> GSSRTSVQTEDDQLIAGQSAGSGSAQLPQEEKAKIAEQVEIFHQEKSKLDAEVAKWDDSGNDIIVLAKQMCMIMMEMTDFTRGKGPLKNTSDVINAAKKIAEAGSRMDKLARA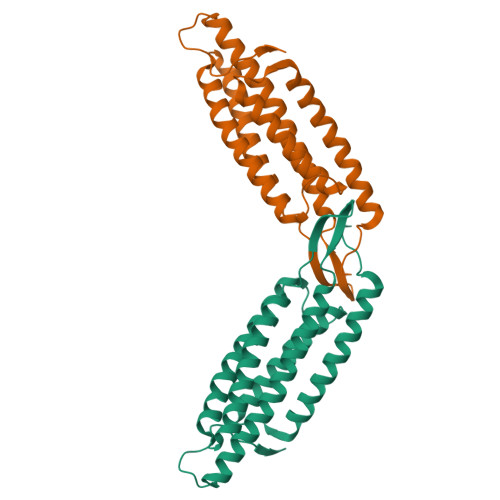VADQCPDSACKQDLLAYLQRIALYCHQLNICSKVKAEVQNLGGELIVSGLDSATSLIQAAKNLMNAVVLTVKASYVASTKYQKVYGTAAVNSPVVSWKMKAPEKKPLVKREKPEEFQTRVRRGSQKKHISPVQALSEFKAMDSF>[2x]MVSYKLTYFNGRGAG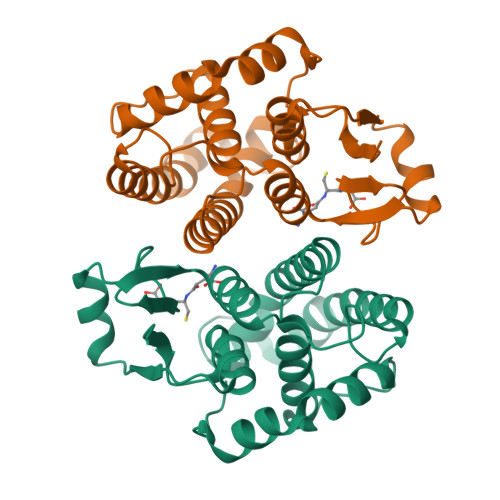EVSRQIFAYAGQQYEDNRVTQEQWPALKETCAAPFGQLPFLEVDGKKLAQSHAIARFLAREFKLNGKTAWEEAQVNSLADQYKDYSSEARPYFYAVMGFGPGDVETLKKDIFLPAFEKFYGFLVNFLKASGSGFLVGDSLTWIDLAIAQHSADLIAKGGDFSKFPELKAHAEKIQAIPQIKKWIETRPVTPF>TIFQFPQDFMWGTATAAYQIEGAYQEDGRGLSIWDTFAHTPGKVFNGDNGNVACDSYHRYEEDIRLMKELGIRTYRFSVSWPRIFPNGDGEVNQKGLDYYHRVVDLLNDNGIEPFCTLYHWDLPQALQDAGGWGNRRTIQAFVQFAETMFREFHGKIQHWLTFNEPWCIAFLSNMLGVHAPGLTNLQTAIDVGHHLLVA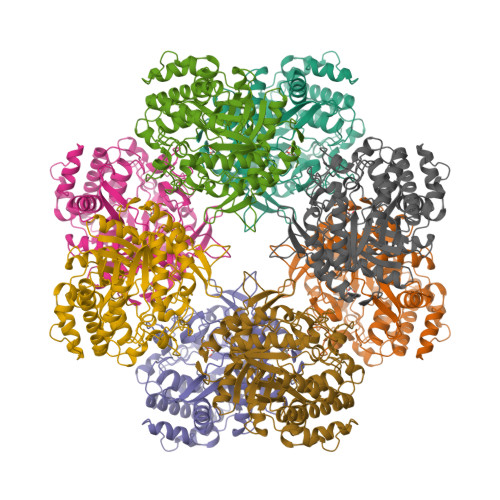HGLSVRRFRELGTSGQIGIAPNVSWAVPYSTSEEDKAACARTISLHSDWFLQPIYQGSYPQFLVDWFAEQGATVPIQDGDMDIIGEPIDMIGINYYSMSVNRFNPEAGFLQSEEINMGLPVTDIGWPVESRGLYEVLHYLQKYGNIDIYITENGACINDEVVNGKVQDDRRISYMQQHLVQVHRTIHDGLHVKGYMAWSLLDNFEWAEGYNMRFGMIHVDFRTQVRTPKESYYWYRNVVSNNWLETRR[4x]>SNAMNYSHPISLKTLVQEDDIGVNAPIIHQSVIARLTAGLYPLYQSKKIPFEPLPETMLTEGYSSPVPDVLLYDHQTEEAKVIIEVCQNSGLKHDTSKIVKLIEDNAYGILEGFVFNYKTQQWLRYRLGDG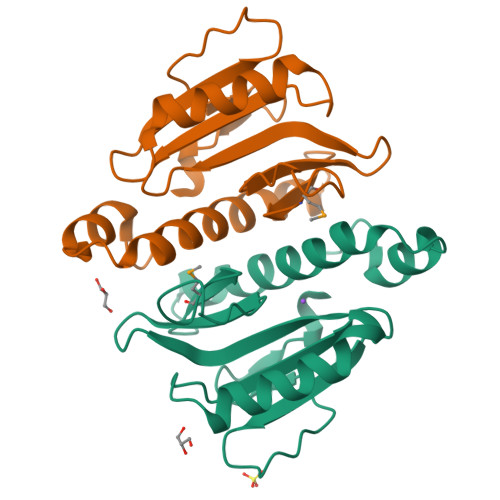GVATNSSFSEVLQVDLNTFV[2x]>MEPSALRKAGSEQEEGFEGLPRRVTDLGMVSNLRRSNSSLFKSWRLQCPFGNNDKQESLSSWIPENIKKKECVYFVESSKLSDAGKVVCQCGYTHEQHLEEATKPHTFQGTQWDPKKHVQEMPTDAFGDIVFTGLSQKVKKYVRVSQDTPSSVIYHLMTQHWGLDVPNLLISVTGGAKNFNMKPRLKSIFRRGLVKVAQTTGAWIITGGSHTGVMKQVGEAVRDFSLSSSYKEGELITIGVATWGTVHRREGLIHPTGSFPAEYILDEDGQGNLTCLDSNHSHFILVDDGTHGQYGVEIPLRTRLEKFISEQTKERGGVAIKIPIVCVVLEGGPGTLHTIDNATTNGTPCVVVEGSGRVADVIAQVANLPVSDITISLIQQKLSVFFQEMFETFTESRIVEWTKKIQDIVRRRQLLTVFREGKDGQQDVDVAILQALLKASRSQDHFGHENWDHQLKLAVAWNRVDIARSEIFMDEWQWKPSDLHPTMTAALISNKPEFVKLFLENGVQLKEFVTWDTLLYLYENLDPSCLFHSKLQKVLVEDPERPACAPAAPRLQMHHVAQVLRELLGDFTQPLYPRPRHNDRLRLLLPVPHVKLNVQGVSLRSLYKRSSGHVTFTMDPIRDLLIWAIVQNRRELAGIIWAQSQDCIAAALACSKILKELSKEEEDTDSSEEMLALAEEYEHRAIGVFTECYRKDEERAQKLLTRVSEAWGKTTCLQLALEAKDMKFVSHGGIQAFLTKVWWGQLSVDNGLWRVTLCMLAFPLLLTGLISFREKRLQDVGTPAARARAFFTAPVVVFHLNILSYFAFLCLFAYVLMVDFQPVPSWCECAIYLWLFSLVCEEMRQLFYDPDECGLMKKAALYFSDFWNKLDVGAILLFVAGLTCRLIPATLYPGRVILSLDFILFCLRLMHIFTISKTLGPKIIIVKRMMKDVFFFLFLLAVWVVSFGVAKQAILIHNERRVDWLFRGAVYHSYLTIFGQIPGYIDGVNFNPEHCSPNGTDPYKPKCPESDATQQRPAFPEWLTVLLLCLYLLFTNILLLNLLIAMFNYTFQQVQEHTDQIWKFQRHDLIEEYHGRPAAPPPFILLSHLQLFIKRVVLKTPAKRHKQLKNKLEKNEEAALLSWEIYLKENYLQNRQFQQKQRPEQKIEDISNKVDAMV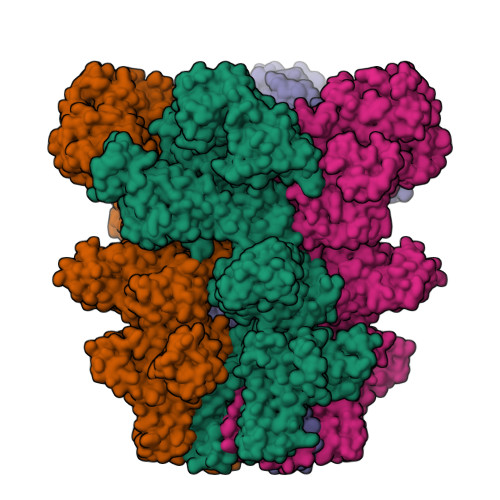DLLDLDPLKRSGSMEQRLASLEEQVAQTAQALHWIVRTLRASGFSSEADVPTLASQKAAEEPDAEPGGRKKTEEPGDSYHVNARHLLYPNCPVTRFPVPNEKVPWETEFLIYDPPFYTAERKDAAAMDPMGDTLEPLSTIQYNVVDGLRDRRSFHGPYTVQAGLPLNPMGRTGLRGRGSLSCFGPNHTLYPMVTRWRRNEDGAICRKSIKKMLEVLVVKLPLSEHWALPGGSREPGEMLPRKLKRILRQEHWPSFENLLKCGMEVYKGYMDDPRNTDNAWIETVAVSVHFQDQNDVELNRLNSNLHACDSGASIRWQVVDRRIPLYANHKTLLQKAAAEFGAHY[4x]>[4x]MVTFLEKISERAKKLN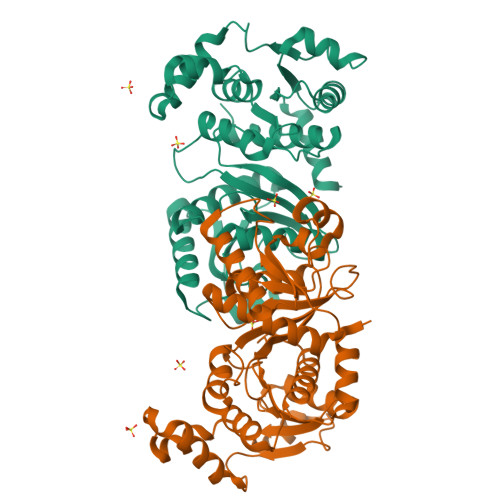KTIALPETEDIRTLQAAAKILERGIADIVLVGNEADIKALAGDLDLSKAKIVDPKTYEKKDEYINAFYELRKHKGITLENAAEIMSDYVYFAVMMAKLGEVDGVVSGAAHSSSDTLRPAVQIVKTAKGAALASAFFIISVPDCEYGSDGTFLFADSGMVEMPSVEDVANIAVISAKTFELLVQDVPKVAMLSYSTKGSAKSKLTEATIASTKLAQELAPDIAIDGELQVDAAIVPKVAASKAPGSPVAGKANVFIFPDLNCGNIAYKIAQRLAKAEAYGPITQGLAKPINDLSRGCSDEDIVGAVAITCVQAAAQDK>[2x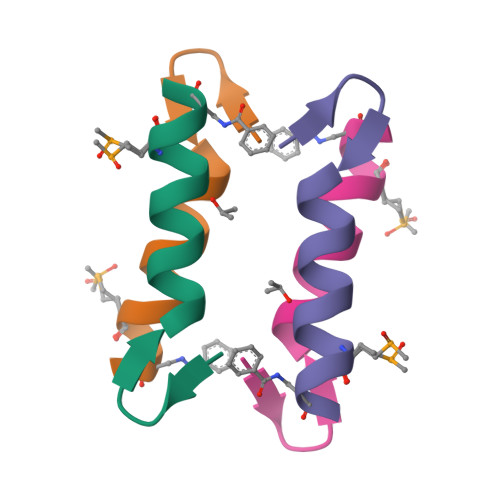]XYRIPSYDFADELAKLLRMAAGX> MDILIVNATDVDEMLKQVEILRRLGAKQIAVVSDDWRILQEALKKGGDILIVNATDVDEMLKQVEILRRLGAKQIAVVSDDWRILQEALKKGGDILIVNATDVDEMLKQVEILRRLGAKQIAVVSDDWRILQEALKKGGDILIVNATDVDEMLKQVEILRRLGAKQIAVVSDD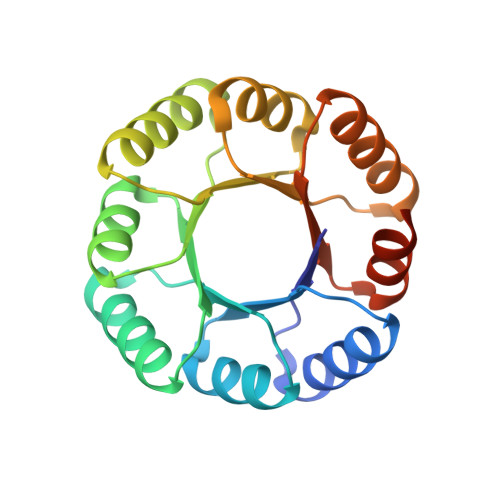WRILQEALKKGGLEHHHHHH> GHMNLPKKVRLVEVGPRDGLQNEKQPIEVADKIRLVDDLSAAGLDYIEVGSFVSPKWVPQMAGSAEVFAGIRQRPGVTYAALAPNLKGFEAALESGVKEVAVFAAASEAFSQRNINCSIKDSLERFVPVLEAARQHQVRVRGYISCVL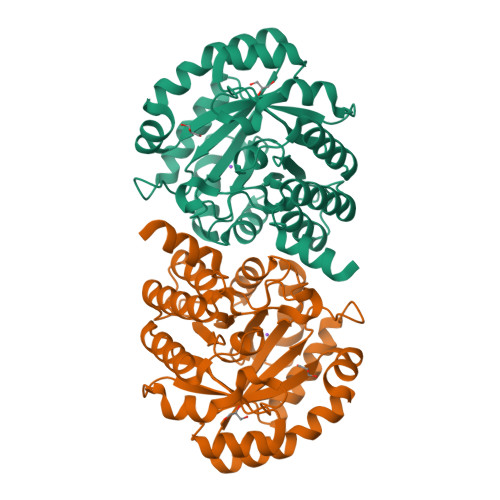GCPYDGDVDPRQVAWVARELQQMGCYEVSLGDTIGVGTAGATRRLIEAVASEVPRERLAGHFHDTYGQALANIYASLLEGIAVFDSSVAGLGGCPYAKGATGNVASEDVLYLLNGLEIHTGVDMHALVDAGQRICAVLGKSNGSRAAKALLAKA> MQNGYTYEDYQDTAKWLLSHTEQRPQVAVICGSGLGGLVNKLTQAQTFDYS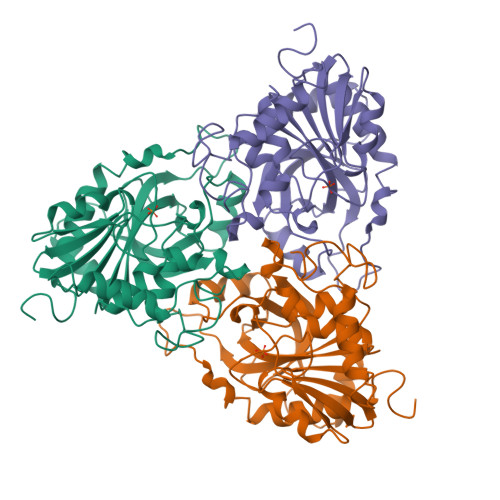EIPNFPESTVPGHAGRLVFGILNGRACVMMQGRFHMYEGYPFWKVTFPVRVFRLLGVETLVVTNAAGGLNPNFEVGDIMLIRDHINLPGFSGENPLRGPNEERFGVRFPAMSDAYDRDMRQKAHSTWKQMGEQRELQEGTYVMLGGPNFETVAECRLLRNLGADAVGMSTVPEVIVARHCGLRVFGFSLITNKVIMDTESQGKANHEEVLEAGKQAAQKLEQFVSLLMASIPVSGHTG> MTIAVTGSIATDHLMRFPGRFSEQLLPEHLHKVSLSFLVDDLVMHRGGVAGNMAFA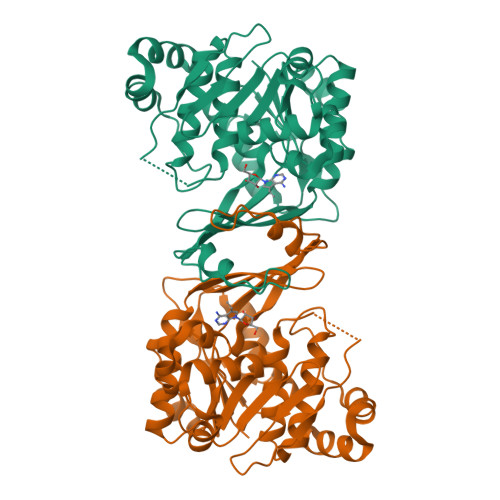IGVLGGEVALVGAAGADFADYRDWLKARGVNCDHVLISETAHTARFTCTTDVDMAQLASFYPGAMSEARNIKLADVVSAIGKPELVIIGANDPEAMFLHTEECRKLGLAFAADPSQQLARLSGEEIRRLVNGAAYLFTNDYEWDLLLSKTGWSEADVMAQIDLRVTTLGPKGVDLVEPDGTTIHVGVVPETSQTDPTGVGDAFRAGFLTGRSAGLGLERSAQLGSLVAVLVLESTGTQEWQWDYEAAASRLAGAYGEHAAAEIVAVLA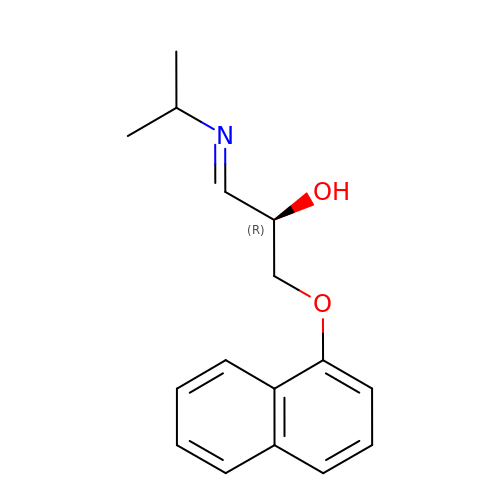(1E,2R)-1-(ISOPROPYLIMINO)-3-(1-NAPHTHYLOXY)PROPAN-2-OL | C16 H19 N O2 | LLOTXRYLQVWOGC-AYCSXLNKSA-N(3S)-3-AMINO-4-PHENYLBUTANOIC ACID | C10 H13 N O2 | 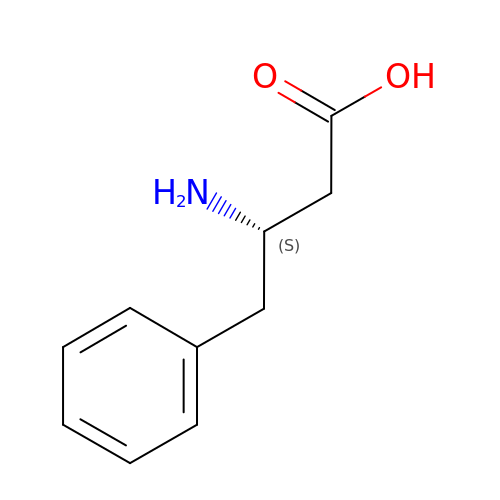OFVBLKINTLPEGH-VIFPVBQESA-N> MAAPAVKSASTPKKATAQFLWEAKTKSGESKKGEMEAMDVEAVNARLKSLGLNPVKVRKKSMLDGDITIPGFGGVEGKDILVFTRQFATMIDAGLPLVQCLDILASQMDNPSFKKVLFAIKSKVEQGSTFADALKEHPKVFDELYVQLCAAGEVGGILDAILNRLAAYREKNEKLKSKV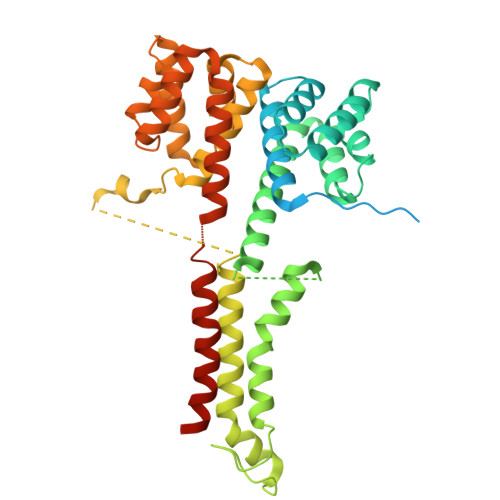KSAMTYPIIVILVAIGVTAVLLLKVTPVFEKMFADFGSELPGPTQMIVNFSHMAQEYFFHVAGSIVAVVMSFTWSYRQPRGRKFWDKVFLFMPVFGPVLRKVAVARFTRTLGTMISSGVPILDALDVTAKTAGNRTVEDAIIYVRGKIAEGKNIAGPLAETKVFPSMVVQMIGVGEATGAMDTMLNKIADFYDDEVDAAINSLTAMIEPVLMVFLGGVVGGFLIGMYLPIFSLAGAIQ>[2x]SVIHYLWVGLPTKMNSSASIAGHDVAGPIKMAKALQSQAQGKPINPIKFWCLEQHQDFYQKLFNDAGVTIEVCGIEEIIRQESQGELRDQALFVQKFLNDNLPSGQNSDIKQRVMFKDLFSLFLLVCQPGYFLDTNVFPATDREINLPGRDTVATAKSGFQ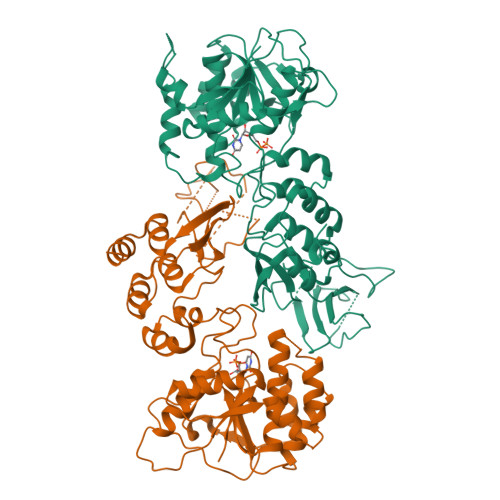KSNDFYLMYSPQRNDSQMSEIFDIWARNPSFGNLLCFSGSHVPYIEIEDLGVQKISYKSYWGAKLPGLFFWLERNNRQLFEENLPYGDINQQLACSFSRKSLAPCSVCYAEEAEPEKLLAMPFTTNEAYIATKANQIFYVNKTTKECVCVSDQFSSLFNCLPDRFHKEKIRLASESEINQLIRSLDNFSHPSYIVNIADGTLLHHAVLSNNIKQVIMLLELGAKFDLKASYQIKPEGTVLKFTPLELANYLKHEAIATLLQSHRI>[2x]MLRKLAAVSLLSLLSAXLLAAECSV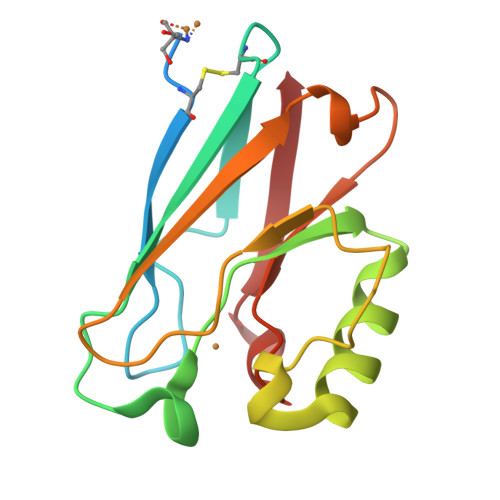DIQGNDQMQFNTNAITVDKSCKQFTVNLSHPGNLPKNVMGHNWVLSTAADMQGVVTDGMASGLDKDFLKPDDSRVIAHTKLIGSGEKDSVTFDVSKLKEGEQFMLFCTFPGHSALMKGTLTLK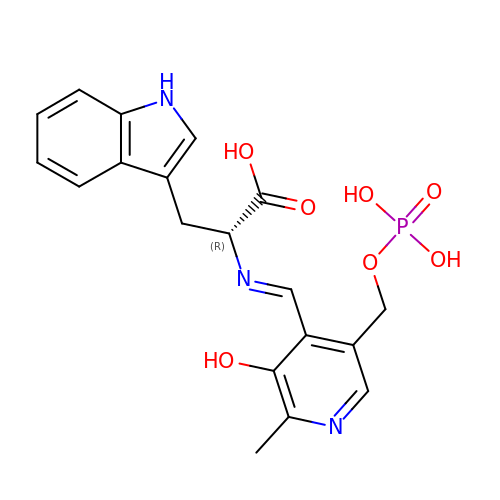(E)-N-({3-hydroxy-2-methyl-5-[(phosphonooxy)methyl]pyridin-4-yl}methylidene)-D-tryptophan | C19 H20 N3 O7 P | MFRRQHVPLFTBMS-KCBMDGGTSA-N> MHHHHHHMSGLSDFFTQLGQDA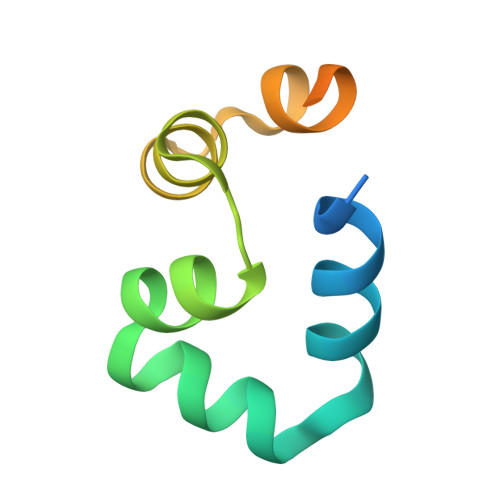QLMEDYKQNPEAVMRAHGLTDEQINAVMTGDMEKLKTLSGDSSYQSALVISHGNGD In bacteria, RuvA, RuvB, and RuvC are involved in processing the HJ. RuvA was shown to assemble into a tetramer for recognizing the HJ core and recruits RuvB. As a motor protein, RuvB can bind the dsDNA part of the HJ and promote the movement of HJ, known as branch migration. RuvB belongs to the AAA+ (ATPase associated with various cellular activities) family, which includes many members involved in numerous physiological processes.

Six RuvB protomers assemble into an asymmetric ring-like hexamer with a 3.0-3.4 nm-wide central pore that accommodates duplex DNA. Strikingly, each protomer (A to F) in the RuvB hexamer adopted a unique conformation. Among the six protomers of the RuvB hexamer, four protomers (A, B, C, and D) assemble into a ‘spiral staircase’ for coordinating dsDNA while the other two protomers (E and F) close the spiral staircase without interacting with DNA substrate. Specifically, three conserved arginine residues R297, R300, and R302 in the RuvB CTD form a motif known as an arginine finger to interact with the negatively charged DNA backbone. R101 next to the Walker B motif and R104 in the β6-β7 loop, two highly conserved residues across species, engaged the backbone of one strand of the dsDNA. Notably, we also noticed that in both DNA-engagement sites, the DNA-interacting arginine residues from protomers B and C are closer to the phosphate backbone than those from protomers A and D, suggesting that protomers B and C engage with DNA more tightly than protomers A and D. In addition, the DNA-engaged arginine residues form a repeated binding pattern along one strand of dsDNA separated by the distance of two nucleotides (about 7 Å), suggesting that the DNA substrate migrates about 7 Å at each step catalyzed by RuvB. Protomers B, C, and D bind ATP molecules while protomers A, F, and E coordinate ADP molecules. Notably, protomer A, located at the top of the staircase, might contain either ADP or ATP with higher occupancy for ADP since ADP can be nicely fitted into the density with a sigma value of 1.8, while ATP can also be nicely placed into the density when we raised the sigma value to 2.5. This observation suggested that ATP hydrolysis occurs at the top of the staircase between protomers A and F. After ATP hydrolysis, the ADP molecules remain associated with RuvB at positions F and E. The ADP to ATP exchange may occur at the position of protomer D as the nucleotide density in protomer D is very poor, likely due to the low occupancy of nucleotides at this position. Therefore, the asymmetric assembly of the RuvB hexamer determines the 6:4 stoichiometry between RuvB and RuvA in the HJ complex.

>[6x]MEDLALRPKTLDEYIGQERLKQKLRVYLEAAKARKEPLEHLLLFGPPGLGKTTLAHVIAHELGVNLRVTSGPAIEKPGDLAAILANSLEEGDILFIDEIHRLSRQAEEHLYPAMEDFVMDIVIGQGPAARTIRLELPRFTLIGATTRPGLITAPLLSRFGIVEHLEYYTPEELAQGVMRDARLLGVRITEEAALEIGRRSRGTMRVAKRLFRRVRDFAQVAGEEVITRERALEALAALGLDELGLEKRDREILEVLILRFGGGPVGLATLATALSEDPGTLEEVHEPYLIRQGLLKRTPRGRVATELAYRHLGYPPPVGPLLEP> MSLQYGAEETPLAGSYGAADSFPKDFGYGVEEEEEEAAAAGGGVGAGAGGGCGPGGADSSKPRILLMGLRRSGKNSIQKVVFHKMSPNETLFLESTNKIYKDDISNSSFVNFQIWDFPGQMDFFDPTFDYEMIFRGTGALIYVIDAQDDYMEALTRLHITVSKAYKVNPDMNFEVFIH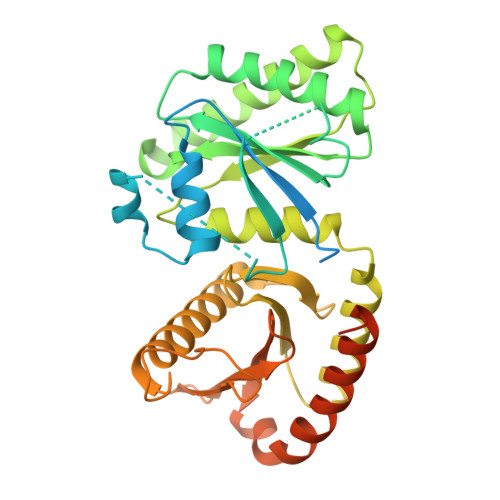KVDGLSDDHKIETQRDIHQRANDDLADAGLEKLHLSFYLTSIYDHSIFEAFSKVVQKLIPQLPTLENLLNIFISNSGIEKAFLFDVVSKIYIATDSSPVDMQSYELCCDMIDVVIDVSCIYGLKEDGSGSAYDKESMAIIKLNNTTVLYLKEVTKFLALVCILREESFERKGLIDYNFHCFRKAIHEVFEVGVTSHRSCGHQTSASSLKALTHNGTPRNAI>MRIIMPVEFSRIVRDVERLIAVEKYSLQGVVDGDKLLVVGFSEGSVNAYLYDGGETVKLNREPINSVLDPHYGVGRVILVRDVSKGAEQHALFKVNTSRPGEEQRLEAVKPMRILSGVDTGEAVVFTGATEDRVALYALDGGGLRELARLPGFGFVSDIRGDLIAGLGFFGGGRVSLFTSNLSSGGLRVFDSGEGSFSSASISPGMKVTAGLETAREARLVTVDPRDGSVEDLE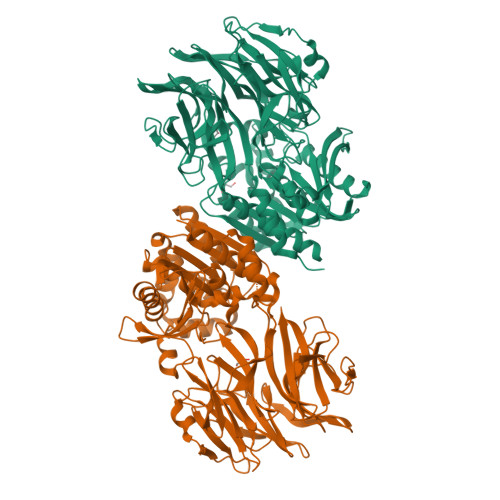LPSKDFSSYRPTAITWLGYLPDGRLAVVARREGRSAVFIDGERVEAPQGNHGRVVLWRGKLVTSHTSLSTPPRIVSLPSGEPLLEGGLPEDLRRSIAGSRLVWVESFDGSRVPTYVLESGRAPTPGPTVVLVHGGPFAEDSDSWDTFAASLAAAGFHVVMPNYRGSTGYGEEWRLKIIGDPCGGELEDVSAAARWARESGLASELYIMGYSYGGYMTLCALTMKPGLFKAGVAGASVVDWEEMYELSDAAFRNFIEQLTGGSREIMRSRSPINHVDRIKEPLALIHPQNDSRTPLKPLLRLMGELLARGKTFEAHIIPDAGHAINTMEDAVKILLPAVFFLATQRERR[4x]>MKEVVIASAVRTAIGSYGKSLKDVPAVDLGATAIKEAVKKAGIKPEDVNEVILGNVLQAGLGQNPARQASFKAGLPQEIPAMTINKVCGSGLRTVSLAAQIIKAGDADVIIAGGMENMSRAPYLANNARWGYRMGNAKFVDEMITDGLWDAFYDYHMGITAENIAERWNISREEQDEFALASQKKAEEAIKSGQFKDEIVPVVIKGRKGETVVDTDEHPRFGSTIEGLAKLKPAFKKDGTVTAGNASGLNDCAAVLVIM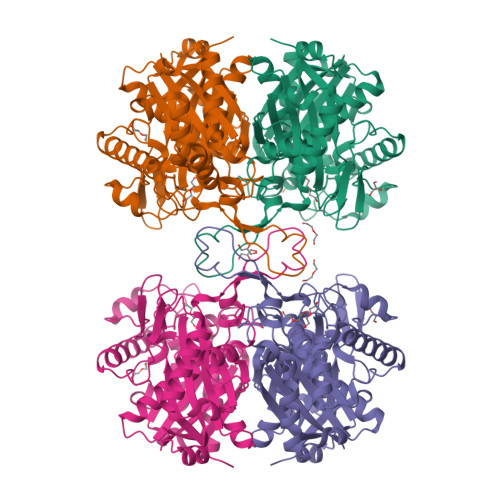SAEKAKELGVKPLAKIVSYGSAGVDPKIMGYGPFYATKAAIEKAGWTVDELDLIESNEAFAAQSLAVAKDLKFDMNKVNVNGGAIALGHPIGASGARILVTLVHAMQKRDAKKGLATLCIGGGQGTAILLEKCLEHHHHHH[2x]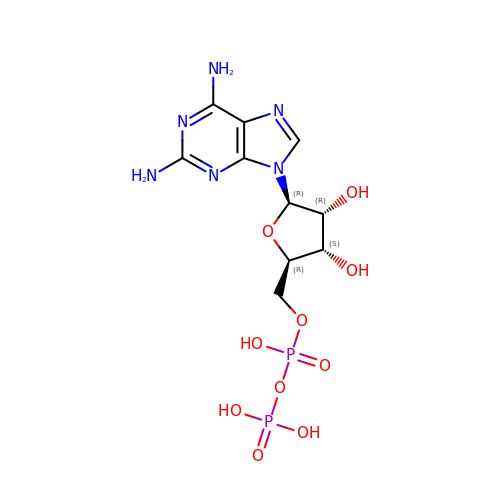[(2~{R},3~{S},4~{R},5~{R})-5-[2,6-bis(azanyl)purin-9-yl]-3,4-bis(oxidanyl)oxolan-2-yl]methyl phosphono hydrogen phosphate | C10 H16 N6 O10 P2 | LOLGBDCHBIGJHI-UUOKFMHZSA-N>[2x]ALYEDPPDQ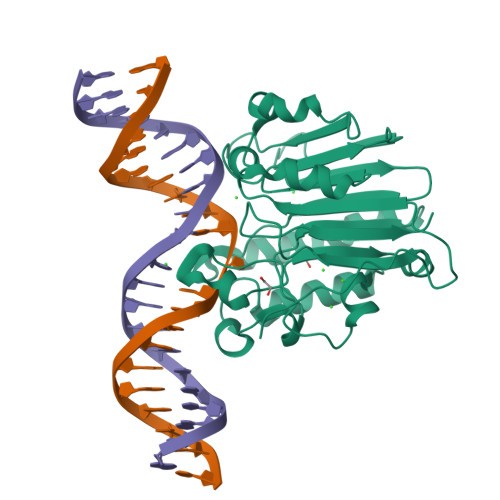KTSPSGKPATLKICSWNVDGLRAWIKKKGLDWVKEEAPDILCLQQTKCSENKLPAELQELPGLSHQYWSAPSDKEGYSGVGLLSRQCPLKVSYGIGDEEHDQEGRVIVAEFDSFVLVTAYVPNAGRGLVRLEYRQRWDEAFRKFLKGLASRKPLVLCGNLNVAHEEIDLRNPKGNKKNAGFTPQERQGFGELLQAVPLADSFRHLYPNTPYAYTFWTYMMNARSKNVGWRLDYFLLSHSLLPALCDSKIRSKALGSDHCPITLYLAL> GSMSEEQVAQDTEEVFRSYVFYRHQQEQEAEGVAAPADPEMVTLPLQPSSTMGQVGRQLAIIGDDINRRYDSEFQTMLQHLQPTAENAYEYFTKIATSLFESGINWGRVVAL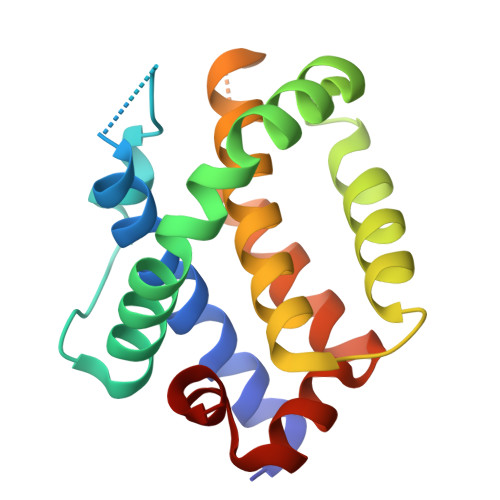LGFGYRLALHVYQHGLTGFLGQVTRFVVDFMLHHSIARWIAQRGGWVAALNL> MTTLLNPYFGEFGGMYVPQILMPALNQLEEAFVSAQKDPEFQAQFADLLKNYAGRPTALTKCQNITAGTRTTLYLKREDLLHGGAHKTNQVLGQALLAKRMGKSEIIAEVGAGNHGVASALASALLGLKCRIYMGAKDVERQSPNVFRMRLMGAEVIPVHSGSATLKDACNEALRDWSGSYETAHYMLGTAAGPHPYPTIVREFQRMIGEETKAQILDKEGRLPDAVIACVGGGSNAIGMFADFINDTSVGLIGVEPGGHGIETGEHGAPLKHGRVGIYFGMKAPMMQTADGQIEESYSISAGLDFPSVGPQHAYLNSIGRADYVSITDDEALEAFKTLCRHEGI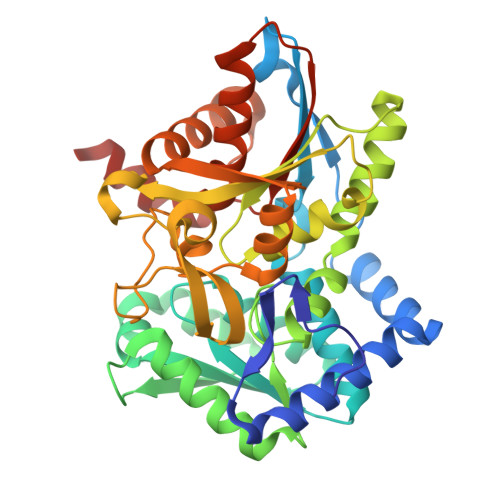IPALESSHALAHALKMMREQPEKEQLLVVNLSGRGDKDIFTVHDILKARGEI> NDPISNAIENAVSTLADTTISRVTAANTAASSHSLGTGRVPALQAAETGASSNASDENLIETRCVMNRNGVNEASVEHFYSRAGLVGVVEVKDSGTSQDGYTVWPIDVMGFVQQRRKLELSTYMRFDAEFTFVSNLNDSTTPGMLLQYMYVPPGAPKPDGRKSYQ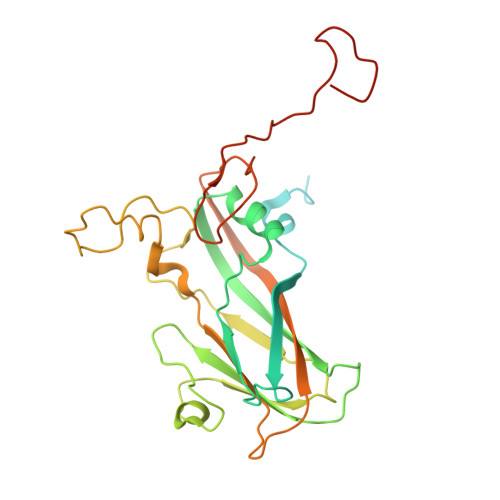WQTATNPSIFAKLSDPPPQVSVPFMSPASAYQWFYDGYPTFGEHKQATNLQYGQCPNNMMGHFAIRTVSESTTGKNVHVRVYMRIKHVRAWVPRPFRSQAYMVKNYPTYSQTISNTAADRASITTTDYEGGVPANPQRTF> SMSLNAADAADERSRKEMDRFQVERMAGQGTFGTVQLGKEKSTGMSVAIKKVIQDPRFRNRELQIMQDLAVLHHPNIVQLQSYFYTLGERDRRDIYLNVVMEYVPDTLHRCCRNYYRRQVAPPPILIKVFLFQLIRSIGCLHLPSVNVCHRDIKPHNVLVNEADGTLKLCDFGSAKKLSPSEPNVAYICSRYYRAPELIFGNQHYTTSVDIWSVGCIFAEMMLGEPIFRGDN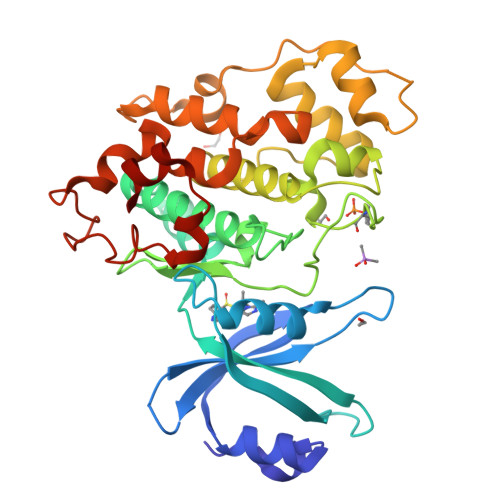SAGQLHEIVRVLGCPSREVLRKLNPSHTDVDLYNSKGIPWSSVFCDHSLKDAKEAYDLLSALLQYLPEDRMKPYEALCHPYFDELHDSATKLPNNKDLPEDLFRFLPSEIEVMSEAQKAKLVRK> LIKHMRAEALFDFTGNSKL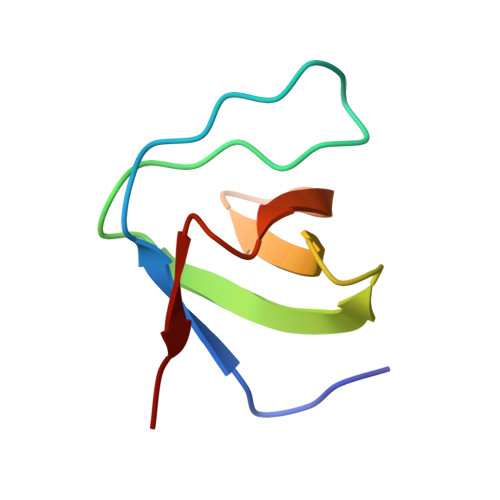ELNFKAGDVIFLLSRINKDWLEGTVRGATGIFPLSFVKILK>[2x]MRSLAILTTLLAGHAFAYPKPAPQSVNRRDWPSINEFLSELAKVMPIGDTITAACDLISDGEDAAASLFGISETENDPCGDVTVLFARGTCDPGNVGVLVGPWFFDSLQTALGSRTLGVKGVPYPASVQDFLSGSVQNGINMANQIKSVLQSCPNTKLVLGGYSQGSMVVHNAASNLDAATMSKISAVVLFGDPYYGKPVANFDAAKTLVVCHDGDNICQGGDIILLPHLTY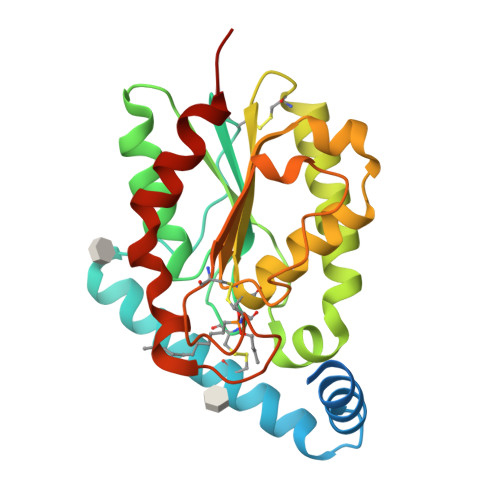AEDADTAAAFVVPLVSHHHHHH7-[(1S)-4-hydroxy-2,3-dihydro-1H-inden-1-yl]-5,5-dimethyl-2-({3-[(pyrrolidin-1-yl)methyl]phenyl}amino)-5,7-dihydro-6H-pyrrolo[2,3-d]pyrimidin-6-one 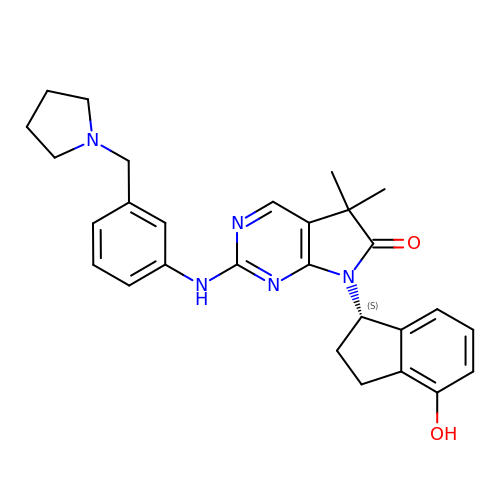| C28 H31 N5 O2 | OFIFLUFVENTCNZ-QHCPKHFHSA-N ARGININE-N-METHYLCARBONYL PHOSPHORIC ACID 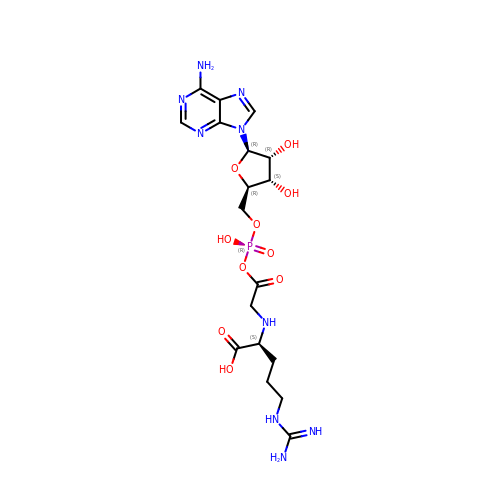5'-ADENOSINE ESTER | C18 H28 N9 O10 P | PLEMKERVZBXYMR-CWPZRQPOSA-N> AKWVYKFEEGNASMRNLLGGKGCNLAEMTILGMPIPQGFTVTTEACTEYYNSGKQITQEIQDQIFEAITWLEELNGKKFGDTEDPLLVSVRSGARASMPGMMDTILNLGLNDVAVEGFAKKTGNPRFAYDSYRRFIQMYSDVVMEVPKSHFEKIIDAMKEEKGVHFDTDLTADDLKELAEKFKAVYKEAMNGEEFPQEPKDQLMGAVKAVFRSWDNPRAIVYRRMNDIPGDWGTAVNVQTMVFGNKGETSGTGVAFTRNPSTGEKGIYGEYLINAQGEDVVAGVRTPQPITQLENDMPDCYKQFMDLAMKLEKHFRDMQDMEFTIEEGKLYFLQTRNGKRTAPAALQIACDLVDEGMITEEEAVVRIEAKSLDQLLHPTFNPAALKAGEVIGSALPASPGAAAGKVYFTADEAKAAHEKGERVILVRLETSPEDIEGMHAAEGILTVRGGMASHAAVVARGMGTCCVSGCGEIKINEEAKTFELGGHTFAEGDYISLDGSTGKIYKGDIETQEASVSGSFERIMVWADKFRTLKVRTNADTPEDTLNAVKLGAEGIGLCRTEHMFFEADRIMKIRKMILSDSVEAREEALNELIPFQKGDFKAMYKALEGRPMTVRYLDPPLHEFVPHTEEEQAELAKNMGLTLAEVKAKVDELHEFNPMMGHRGCRLAVTYPEIAKMQTRAVMEAAIEVKEETGIDIVPEIMIPLVGEKKELKFVKDVVVEVAEQVKKEKGSDMQYHIGTMIEIPRAALTADAIAEEAEFFSFGTNDLTQMTFGFSRDDAGKFLDSYYKAKIYESDPFARLDQTGVGQLVEMAVKKGRQTRPGLKCGICGEHGGDPSSVEFCHKVGLNYVS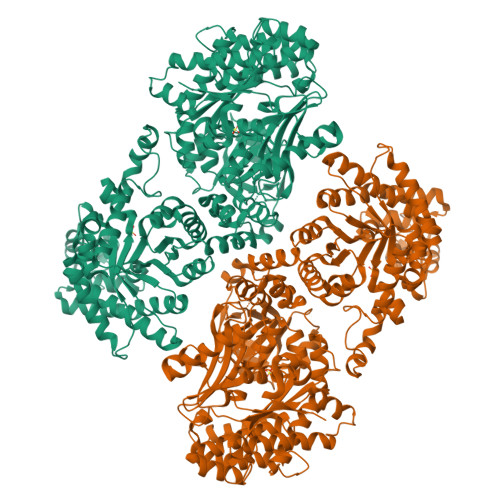CSPFRVPIARLAAAQAALNNK>[2x]AEPVYPDQLRLFSLGQGVCGDKYRPVNREEAQSVKSNIVGMMGQWQISGLANGWVIMGPGYNGEIKPGTASNTWCYPTNPVTGEIPTLSALDIPDGDEVDVQWRLVHDSANFIKPTSYLAHYLGYAWVGGNNSQYVGEDMDVTRDGDGWVIRGNNDGGCDGYRCGDKTAIKVSNFAYNLDPDSFKHGD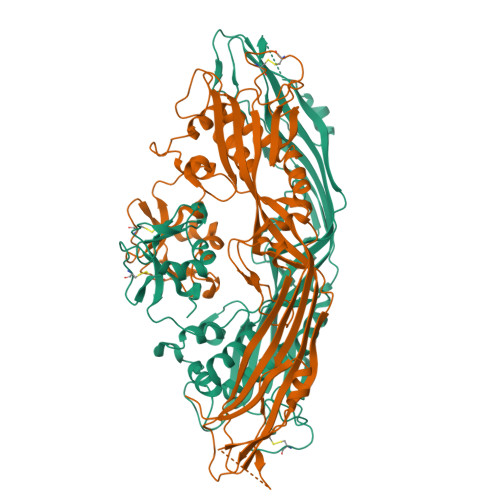VTQSDRQLVKTVVGWAVNDSDTPQSGYDVTLRYDTATNWSKTNTYGLSEKVTTKNKFKWPLVGETELSIEIAANQSWASQNGGSTTTSLSQSVRPTVPARSKIPVKIELYKADISYPYEFKADVSYDLTLSGFLRWGGNAWYTHPDNRPNWNHTFVIGPYKDKASSIRYQWDKRYIPGEVKWWDWNWTIQQNGLSTMQNNLARVLRPVRAGITGDFSAESQFAGNIEIGAPVPLAADSKVRRARSVDGAGQGLRLEIPLDAQELSGLGFNNVSLSVTPAANQ> HI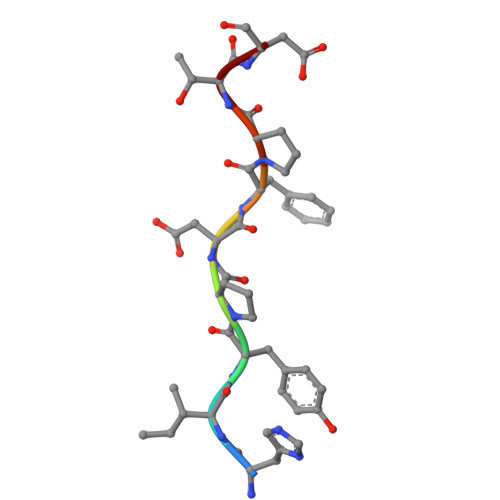YPDFPTD> TSRRPRLAPPQNVTLLSQNFSVYLTWLPGLGNPQDVTYFVAYQSSPTRRRWREVEECAGTKELLCSMMCLKKQDLYNKFKGRVRTVSPSSKSPWVE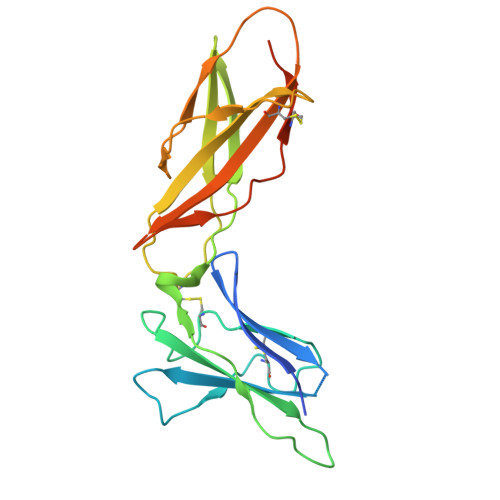SEYLDYLFEVEPAPPVLVLTQTEEILSANATYQLPPCMPPLDLKYEVAFWKEGAGNKTLFPVTPHGQPVQITLQPAASEHHCLSARTIYTFSVPKYSKFSKPTCFLLEVPEANAAALEVLFQ>[4x]SAQVGTNKELCCLVYTSWQIPQKFIVDYSETSPQCPKPGVILLTKRGRQICADPNKKWVQKYISDLKLNA

CC chemokine ligands (CCL) comprise 8-14 kDa chemotactic cytokines (chemokines) involved in diverse immune functions. Extensive structural analyses reveal that most chemokines share a common core structure: an N-terminal extension followed by a 310 helical turn, an anti-parallel three-stranded β-sheet, and an α-helix. CC chemokines also readily dimerize, primarily through the formation of an anti-parallel β-sheet at their N-termini. Certain chemokines, e.g. CCL3, CCL4, and CCL5 form polydisperse, high MW reversible polymers in excess of 600 kDa without the assistance of GAG.

CCL18, also known as pulmonary and activation regulated chemokine (PARC) among other names (e.g., MIP-4, DC-CK1, and AMAC-1), is a primate-specific CC chemokine expressed by macrophages, monocytes, and dendritic cells upon infection or inflammation to attract T cells. We next found diffraction-quality crystals in the presence of citrate ion via a high-throughput sparse matrix method and solved the structure of CCL18 at 2.1Å resolution in space group P21. There are two CCL18 dimers in each asymmetric unit. The overall CCL18 monomer structure consists of an N-terminal segment (aa 1-21) followed by a 310 helical turn (aa 22-24), an anti-parallel three-stranded β-sheet (aa 25-56), and an α-helix (aa 56-69). The two monomers within the CCL18 dimer adopt distinct structures at their N-termini; one has the N-terminal extension (aa 1-6) followed by an α-helix (aa 7-10) and the other has a largely disordered N-terminus (aa 1-7). The N-termini of these two monomers (aa 2-5 in one and aa 8-13 in the other) form a network of hydrogen bonds and van der Waal contacts between their N-termini that bury a substantial surface (~549 Å2). The dimer contacts of CCL18 are distinct from other CCL dimers, which form contacts at their N-terminal region via an anti-parallel β-sheet, exemplified by CCL3. We find that the N-terminus of a CCL18 monomer within CCL18 dimer adopts α-helical conformation, which is distinct from the typical anti-parallel β-sheet shown in the other CCL dimers. Such an interface weakens the interaction between CCL18 monomers, explaining why CCL18 prefers the monomeric state in solution. Examining the contacts between the symmetry-related CCL18 in our CCL18 structure reveals a 630 Å2 buried surface. This permits the formation of a CCL18 oligomer that can be extended at either end in a zigzag manner.> MYKNIEDLNKFASKILETEISFEESITFTPDEVEENIGEKPNRDKICHSTSLEDGRVIML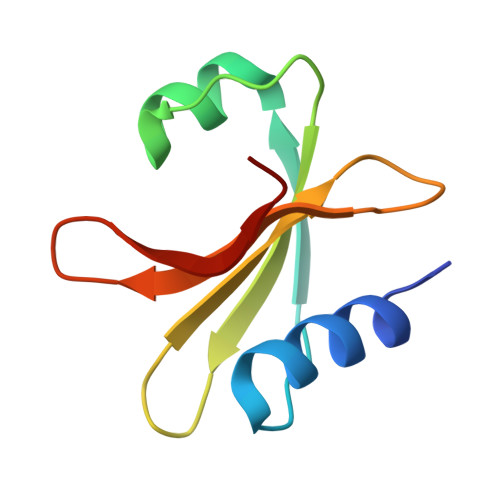LTELEPNYTPWKLLELEEDGFKELYSKSI In addition to the shared TMD-DH catalytic core of NOX, the functional DUOX protein has an additional large N-terminal extracellular peroxidase homology domain (PHD) and a long intracellular loop 0 containing two EF-hand domains, and it requires an auxiliary DUOXA protein for proper function. The activity of DUOX is regulated by intracellular calcium concentration. hDUOX1 subunits and hDUOXA1 subunits co-assemble into a 2:2 heterotetrameric protein complex with molecular weight ~457 kDa. Here, we present the cryo-EM structures of human DUOX1–DUOXA1 (hDUOX1–hDUOXA1) complex in both high-calcium and low-calcium states, providing insights into the structure and mechanism of calcium activation for DUOX.

In the low-calcium condition, DUOX1–DUOXA1 complex showed low basal activity. We compared the structures in the low-calcium state and high-calcium state, and found structural changes in the extracellular layer and transmembrane layer are small. However, there are large conformational changes of the regulatory PHLD and EF-hand module in the cytosolic layer. In the absence of calcium, the EF module switches from an extended shape into a more contracted shape, which reconfigures the interface between the EF module and α4 of the DH domain, resulting in a loosely packed structure. In the low-calcium state, EF2 moves away from the DH domain. The Cα atom of A894 on αJ of EF2 has 40 Å displacement. PHLD rotates away from the TMD and DH domains, and αA of PHLD has 17.2° outward rotation. As a result, several inter-domain interactions observed in the high-calcium state were disrupted and therefore the docking of DH domain onto TMD is weakened by these structural changes, leading to a higher mobility of DH domain. We propose the increased mobility of DH domain negatively correlates with the electron transfer efficiency and thus the catalytic activity of DUOX. Removal of calcium ions results in the reconfiguration of cytosolic inter-domain interactions which in turn mobilizes the DH domain and lowers the electron transfer efficiency.

>MGFCLALAWTLLVGAWTPLGAQNPISWEVQRFDGWYNNLMEHRWGSKGSRLQRLVPASYADGVYQPLGEPHLPNPRDLSNTISRGPAGLASLRNRTVLGVFFGYHVLSDLVSVETPGCPAEFLNIRIPPGDPMFDPDQRGDVVLPFQRSRWDPETGRSPSNPRDPANQVTGWLDGSAIYGSSHSWSDALRSFSRGQLASGPDPAFPRDSQNPLLMWAAPDPATGQNGPRGLYAFGAERGNREPFLQALGLLWFRYHNLWAQRLARQHPDWEDEELFQHARKRVIATYQNIAVYEWLPSFLQKTLPEYTGYRPFLDPSISSEFVAASEQFLSTMVPPGVYMRNASCHFQGVINRNSSVSRALRVCNSYWSREHPSLQSAEDVDALLLGMASQIAEREDHVLVEDVRDFWPGPLKFSRTDHLASCLQRGRDLGLPSYTKARAALGLSPITRWQDINPALSRSNDTVLEATAALYNQDLSWLELLPGGLLESHRDPGPLFSTIVLEQFVRLRDGDRYWFENTRNGLFSKKEIEEIRNTTLQDVLVAVINIDPSALQPNVFVWHKGDPCPQPRQLSTEGLPACAPSVVRDYFEGSGFGFGVTIGTLCCFPLVSLLSAWIVARLRMRNFKRLQGQDRQSIVSEKLVGGMEALEWQGHKEPCRPVLVYLQPGQIRVVDGRLTVLRTIQLQPPQKVNFVLSSNRGRRTLLLKIPKEYDLVLLFNLEEERQALVENLRGALKESGLSIQEWELREQELMRAAVTREQRRHLLETFFRHLFSQVLDINQADAGTLPLDSSQKVREALTCELSRAEFAESLGLKPQDMFVESMFSLADKDGNGYLSFREFLDILVVFMKGSPEEKSRLMFRMYDFDGNGLISKDEFIRMLRSFIEISNNCLSKAQLAEVVESMFRESGFQDKEELTWEDFHFMLRDHNSELRFTQLCVKGVEVPEVIKDLCRRASYISQDMICPSPRVSARCSRSDIETELTPQRLQCPMDTDPPQEIRRRFGKKVTSFQPLLFTEAHREKFQRSCLHQTVQQFKRFIENYRRHIGCVAVFYAIAGGLFLERAYYYAFAAHHTGITDTTRVGIILSRGTAASISFMFSYILLTMCRNLITFLRETFLNRYVPFDAAVDFHRLIASTAIVLTVLHSVGHVVNVYLFSISPLSVLSCLFPGLFHDDGSEFPQKYYWWFFQTVPGLTGVVLLLILAIMYVFASHHFRRRSFRGFWLTHHLYILLYVLLIIHGSFALIQLPRFHIFFLVPAIIYGGDKLVSLSRKKVEISVVKAELLPSGVTHLRFQRPQGFEYKSGQWVRIACLALGTTEYHPFTLTSAPHEDTLSLHIRAAGPWTTRLREIYSAPTGDRCARYPKLYLDGPFGEGHQEWHKFEVSVLVGGGIGVTPFASILKDLVFKSSVSCQVFCKKIYFIWVTRTQRQFEWLADIIREVEENDHQDLVSVHIYITQLAEKFDLRTTMLYICERHFQKVLNRSLFTGLRSITHFGRPPFEPFFNSLQEVHPQVRKIGVFSCGPPGMTKNVEKACQLINRQDRTHFSHHYENF[2x];>MATLGHTFPFYAGPKPTFPMDTTLASIIMIFLTALATFIVILPGIRGKTRLFWLLRVVTSLFIGAAILAVNFSSEWSVGQVSTNTSYKAFSSEWISADIGLQVGLGGVNITLTGTPVQQLNETINYNEEFTWRLGENYAEEYAKALEKGLPDPVLYLAEKFTPRSPCGLYRQYRLAGHYTSAMLWVAFLCWLLANVMLSMPVLVYGGYMLLATGIFQLLALLFFSMATSLTSPCPLHLGASVLHTHHGPAFWITLTTGLLCVLLGLAMAVAHRMQPHRLKAFFNQSVDEDPMLEWSPEEGGLLSPRYRSMADSPKSQDIPLSEASSTKAYYRPRRLSLVPADVRGLAPAALSALPGALLAQAWRALLPGLRCPKAGKESRLGPPHSPWRFGPEGCEERWAEHTGDSPRPLRGRGTGRLWRWGSKERRACGVRAMLPRLVSNSGLKRPSCLDLPKCWDYRRDARAFFHLLEPTPCVTSRHTPLI[2x]> MESKKRQWALEDFEIGRPLGKGKFGNVYLAREKQSKFILALKVLFKAQLEKAGVEHQLRREVEIQSHLRHPNILRLYGYFHDATRVYLILEYAPLGTVYRELQKLSKFDEQRTATYITELANALSYCHSKRVIHRDIKPENLLLGSAGELKIANFGWSVHA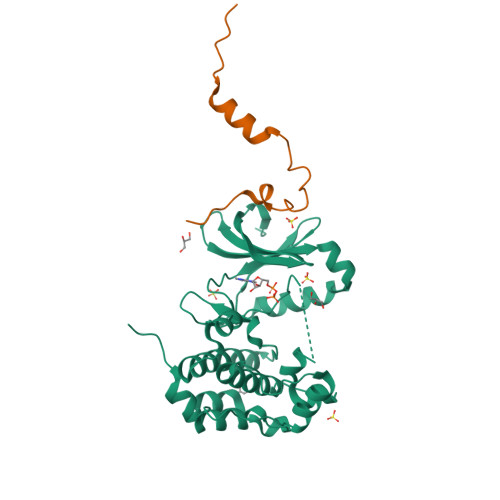PSSRRTTLAGTLDYLPPEMIEGRMHDEKVDLWSLGVLCYEFLVGKPPFEANTYQETYKRISRVEFTFPDFVTEGARDLISRLLKHNPSQRPMLREVLEHPWITANSSKPSNAQNKESASKQS;> MELKEESFRDPAEVLGTGAEVDYLEQFGTSSFKESALRKQSLYLKF>[2x]XAATSRPERVWPDGVIPFVIGGNFTGSQRAVFRQAMRHWEKHTCVTFLERTDEDSYIVFTYRPCGCCSYVGRRGGGPQAISIGKNCDKFGIVVHELGHVVGFWHEHTRPDRDRHVSI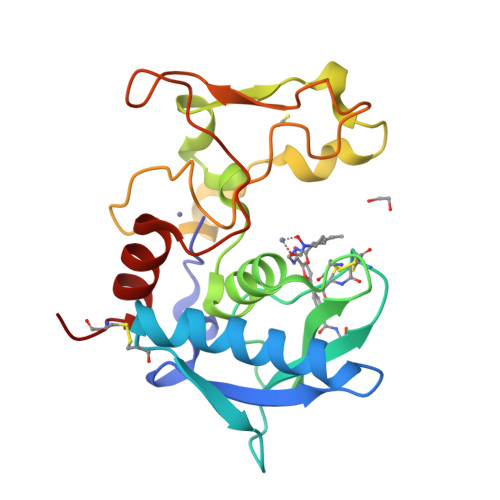VRENIQPGQEYNFLKMEPQEVESLGETYDFDSIMHYARNTFSRGIFLDTIVPKYEVNGVKPPIGQRTRLSKGDIAQARKLYKCPA>MAHHHHHHVGTMSNTGFYTHESTFWHSTGVQALYFPIGEWVQPPSGTYGADTPETKRRFLNLLRMSGLTDRLVMPAGEPVTVEDCLRIHPADYIRRFKEASDAGGGDLGMLAPFSKGGFEIALMSAGLARAAIDDVLTGKVRNAYALSRPAGHHCLPDTPMGFCLLANIPIAIEAARARHGIERVAVVDWDVHHGNGTQACYYDRSDVLTISVHQDRCFPPGYSGVEERGEGAGLGHNINIPLPAGSGQDTYVHAFETIVLPALDRYRPDLIVVASGLDANAVDPLARMLLFSESYRVLTGMMMDAADRLCEGRLAVVHEGGYSEAYVPFCGQAIVETLAGVRTGVVDPELEMFALWQPGDRINRFHRELVDEMAAVLLG[8x]

Classical Zn2+-dependent deac(et)ylases play fundamental regulatory roles in life and are well characterized in eukaryotes regarding their structures, substrates and physiological roles. Structurally, these enzymes are composed of a central eight-stranded parallel β-sheet flanked by α-helices on each site, known as the α/β-arginase/deacetylase fold. All active site residues were conserved, as shown by the multiple sequence alignment and the structural alignment, suggesting a general acid/base catalytic mechanism for the bacterial enzymes as described for the eukaryotic counterparts. These enzymes mediate catalysis using a penta-coordinated catalytic Zn2+ ion coordinated by two aspartates and a histidine (KpHdaH (1b): Asp181, Asp269, His183).

We solved the crystal structures of three enzymes representing cluster 1 amidohydrolases: KpHdaH (1b), RwDmhA (1b), and RsPrpH (1b). This cluster contains enzymes with efficient lysine deacetylase activity, but also evolutionary divergent enzymes as RwDmhA (1b) and RsPrpH (1b) developed to be active as small molecule amidohydrolases. For RsPrpH (1b) acting as arylamidase converting the pesticide propanil to 3,4-dichloraniline rather than lysine deacetylase. RsPrpH (1b) was isolated from wastewater showing activity as propanil hydrolase for which Zn2+ has inhibitory potential. For the cluster 1b enzyme RsPrpH (1b) the deacylase activity was almost nondetectable, only for the H3-derived peptide APRKac we observed a weak deacetylase activity. Only for RwDmhA (1b) and RsPrpH (1b), which evolved toward non-protein substrates, the second proline is substituted for an Ala suggesting this position being important for substrate specificity to accommodate the product. For RwDmhA (1b) and RsPrpH (1b) we discovered a hydrophobic 22-LFL-24/32-LYF-34 motif in the L1-loop lining the substrate binding tunnel, the sequence 98-GHLAP-102/107-GMLAP-111 as well as the sequence 342-MAEAW-346/352-MFALW−356 in the C-terminal α-helix lining the active site rim. Notably, for all sub-cluster 1b enzymes, except for RwDmhA (1b), we found an acetate molecule in the active site coordinating the active site Zn2+ ion. For RsPrpH (1b) and RwDmhA (1b) the data suggest that these enzymes represent examples for divergent evolution developing toward an activity to convert specific substrates, i.e. propanil or dimethoate, while losing their efficiency to deacetylate lysine side chains, supporting that enzymes with different activities might be present within a cluster. For RwDmhA (1b) and RsPrpH (1b), we characterized two examples of deacetylases that divergently evolved from protein lysine deacetylases to enzymes with substrate specificity for small molecules, i.e. dimethoate and propanil.>[2x]GPLGMAGLGHPAAFGRATHAVVRALPESLGQHALRSAKGEEVDVARAERQHQLYVGVLGSKLGLQVVELPADESLPDCVFVEDVAVVCEETALI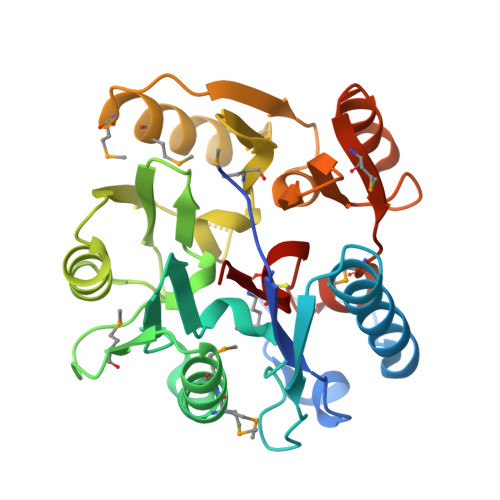TRPGAPSRRKEVDMMKEALEKLQLNIVEMKDENATLDGGDVLFTGREFFVGLSKRTNQRGAEILADTFKDYAVSTVPVADGLHLKSFCSMAGPNLIAIGSSESAQKALKIMQQMSDHRYDKLTVPDDIAANCIYLNIPNKGHVLLHRTPEEYPESAKVYEKLKDHMLIPVSMSELEKVDGLLTCCSVLINKKVDS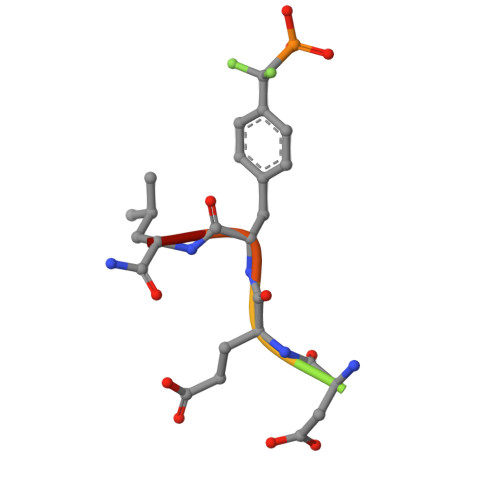> DADEYLX>[2x]ARTVVLITGCSSGIGLHLAVRLASDPSQSFKVYATLRDLKTQGRLWEAARALACPPGSLETLQLDVRDSKSVAAARERVTEGRVDVLVCNAGLGLLGPLEALGEDAVASVLDVNVVGTVRMLQAFLPDMKRRGSGRVLVTGSVGGLMGLPFNDVYCASKFALEGLCESLAVLLLPFGVHLSL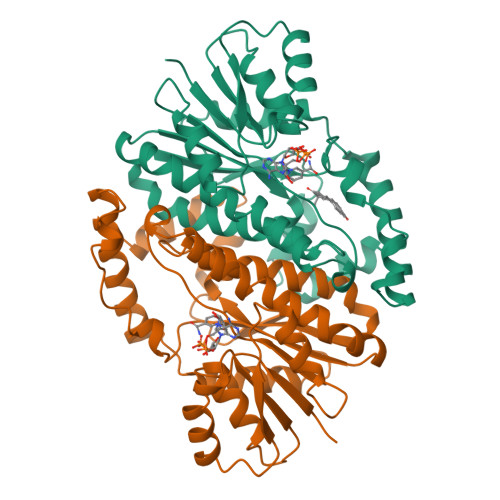IECGPVHTAFMEKVLGSPEEVLDRTDIHTFHRFYQYLAHSKQVFREAAQNPEEVAEVFLTALRAPKPTLRYFTTERFLPLLRMRLDDPSGSNYVTAMHREVFGDVPAKAEAGAEAGGGAGPGAEDEAGRSAVGDPELGDPPAAPQ> MSASSERELYEAWVELLSWMREYAQAKGVRFEKEADFPDFIYRMERPYDLPTTIMTASLSDGLGEPFLLADVSPRHAKLK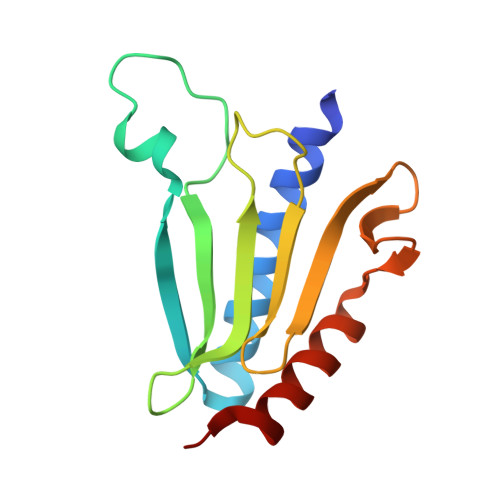RIGLRLPRAHIHLHAHYEPGKGLVTGKIPLTKERFFALADRAREALAFA>[4x]GPHMDVHEIDETLEKFLAENYTPERVQQLADRFQRTGFVKFDSHMRIVPEELITAVRAEADRLVREHKERRDLVLGTTGGTPRNLSVVKSQDVEQSDLIRAVTRSEVLLTFLAGITRERIIPEVSDDERYLITHQEFASDTHGWHWDDYSFAF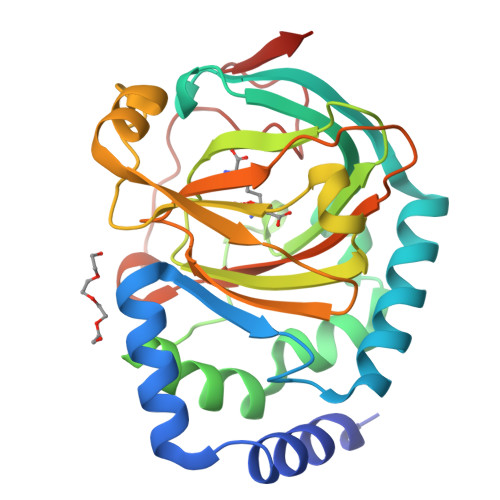NWALRMPPIASGGMVQAVPHTHWDKNAPRINETLCERQIDTYGLVSGDLYLLRSDTTMHRTVPLTEDGAVRTMLVVSWSAERDLGKVLTGNDRWWENPEAGAAQPVHRAG> MKIVIVKKVEIQVAGRTGMRCAS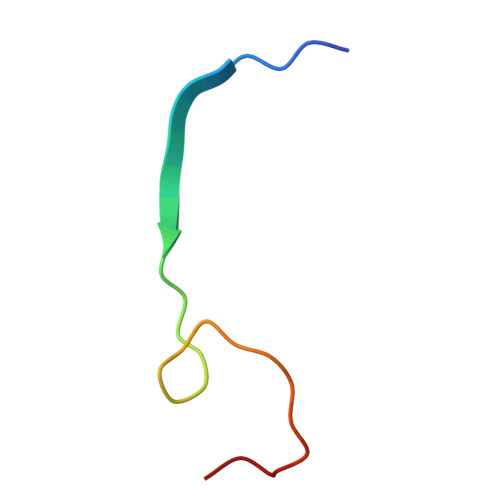SCGAKS>GSHMTYRDAATALEHLATYAEKDGLSVEQLMDSKTRGGLTYNDFLVLPGKIDFPSSEVVLSSRLTKKITLNAPFVSSPMDTVTEADMAIHMALLGGIGIIHHNCTAEEQAEMVRRVKKYENGSQDGPLASKSADTKQLLCGAAIGTIDADRQRLAMLVEAGLDVVVLDSSQGNSVFQINMIKWIKETFPDLQVIAGNVVTREQAASLIHAGADGLRIGMGSGSICITQEVMACGRPQGTAVYNVTQFANQFGVPCIADGGVQNIGHITKAIALGASTVMMGGMLAGTTESPGEYFFRDGKRLKTYRGMGSID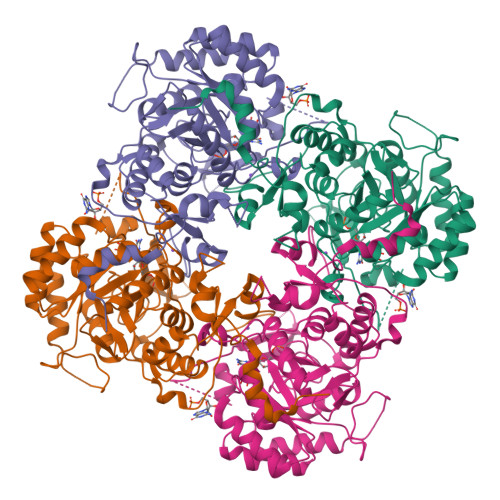AMQKTDVKGNAATSRYFSESDKVLVAQGVTGSVIDKGSIKKYIPYLYNGLQHSCQDIGVRSLVEFREKVDSGSVRFEFRTPSAQLEGGVHNLHSYEKRLFD[2x]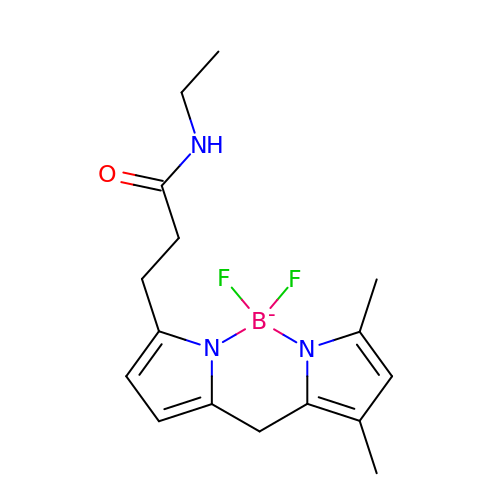3-[2,2-bis(fluoranyl)-10,12-dimethyl-1,3-diaza-2$l^{4}-boratricyclo[7.3.0.0^{3,7}]dodeca-4,6,9,11-tetraen-4-yl]-~{N}-ethyl-propanamide | C16 H21 B F2 N3 O | QWVZNTQOZDNYPL-UHFFFAOYSA-N> GCMNGGGDLAGKWQLRQYQYADGTSEKVDSVFYNFQKGS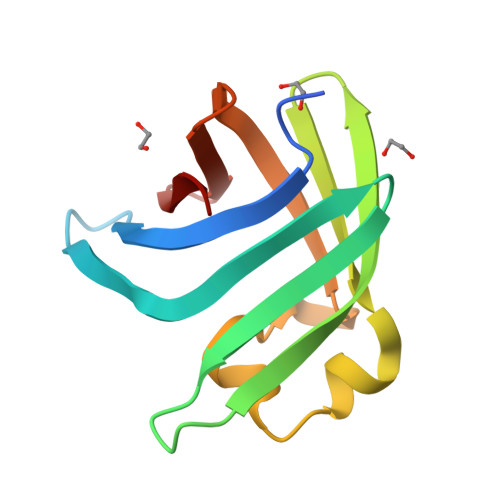FSAICLLKDGGLTTFFGNYSLKGAEISIILLPESVNDKNYDTYFGWPEGKCTFKVEDLSYSSLRLEYEGTKSIFRKF> ELHIGGIFPIAGKGGWQGGQACMPATRLALDDVNKQPNLLPGFKLILHSNDSECEPGLGASVMYNLLYNKPQKLMLLAGCSTVCTTVAEAAKMWNLIVLCYGASSPALSDRKRFPTLFRTHPSATVHNPTRIKLMKKFGWSRVAILQQAEEVFISTVEDLENRCMEAGVEIVTRQSFLSDPTDAVRNLRRQDARIIVGLFYVVAARRVLCEMYKQQLYGRAHVWFFIGWYEDNWYEVNLKAEGITCTVEQMRIAAEGHLTTEALMWNQNNQTTISGMTAEEFRHRLNQALIEEGYDINHDRYPEGYQEAPLAYDAVWSVALAFNKTME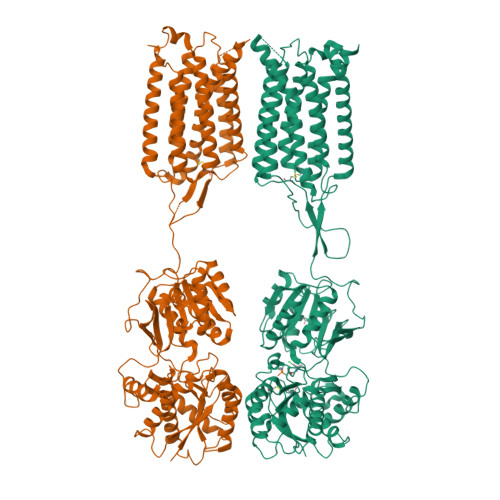RLTTGKKSLRDFTYTDKEIADEIYAAMNSTQFLGVSGVVAFSSQGDRIALTQIEQMIDGKYEKLGYYDTQLDNLSWLNTEQWIGGKVPQDRTIVTHVLRTVSLPLFVCMCTISSCGIFVAFALIIFNIWNKHRRVIQSSHPVCNTIMLFGVIICLISVILLGIDGRFVSPEEYPKICQARAWLLSTGFTLAYGAMFSKVWRVHRFTTKAKTDPKKKVEPWKLYTMVSGLLSIDLVILLSWQIFDPLQRYLETFPLEDPVSTTDDIKIRPELEHCESQRNSMWLGLVYGFKGLILVFGLFLAYETRSIKVKQINDSRYVGMSIYNVVVLCLITAPVGMVIASQQDASFAFVALAVIFCCFLSMLLIFVPKVIEVIRH;> RTAKRSDVYIAGFFPYGDGVENSYTGRGVMPSVKLALGHVNEHGKILANYRLHMWWNDTQCNAAVGVKSFFDMMHSGPNKVMLFGAACTHVTDPIAKASKHWHLTQLSYADTHPMFTKDAFPNFFRVVPSENAFNAPRLALLKEFNWTRVGTVYQNEPRYSLPHNHMVADLDAMEVEVVETQSFVNDVAESLKKLREKDVRIILGNFNEHFARKAFCEAYKLDMYGRAYQWLIMATYSTDWWNVTQDSECSVEEIATALEGAILVDLLPLSTSGDITVAGITADEYLVEYDRLRGTEYSRFHGYTYDGIWAAALAIQYVAEKREDLLTHFDYRVKDWESVFLEALRNTSFEGVTGPVRFYNNERKANILINQFQLGQMEKIGEYHSQKSHLDLSLGKPVKWVGKTPPKDRTLIYIEHSQVNPTIYIVSASASVIGVIIATVFLAFNIKYRNQRYIKMSSPHLNNLIIVGCMITYLSIIFLGLDTTLSSVAAFPYICTARAWILMAGFSLSFGAMFSKTWRVHSIFTDLKLNKKVIKDYQLFMVVGVLLAIDIAIITTWQIADPFYRETKQLEPLHHENIDDVLVIPENEYCQSEHMTIFVSIIYAYKGLLLVFGAFLAWETRHVSIPALNDSKHIGFSVYNVFITCLAGAAISLVLSDRKDLVFVLLSFFIIFCTTATLCLVFVPKLVELKRNPQGVVDKRVRATLRPMSKNGRRDSSVCELEQRLRDVKNTNCRFRKALMEKENELQALIRKLGPEARKWIDGVTC> SAPGEDEECGRVRDFVAKLANNTHQHVFDDLRGSVSLSWVGDSTGVILVLTTFHVPLVIMTFGQSKLYRSEDYGKNFKDITDLINNTFIRTEFGMAIGPENSGKVVLTAEVSGGSRGGRIFRSSDFAKNFVQTDLPFHPLTQMMYSPQNSDYLLALSTENGLWVSKNFGGKWEEIHKAVCLAKWGSDNTIFFTTYANGSCKADLGALELWRTSDLGKSFKTIGVKIYSFGLGGRFLFASVMADKDTTRRIHVSTDQGDTWSMAQLPSVGQEQFYSILAANDDMVFMHVDEPGDTGFGTIFTSDDRGIVYSKSLDRHLYTTTGGETDFTNVTSLRGVYITSVLSEDNSIQTMITFDQGGRWTHLRKPENSECDA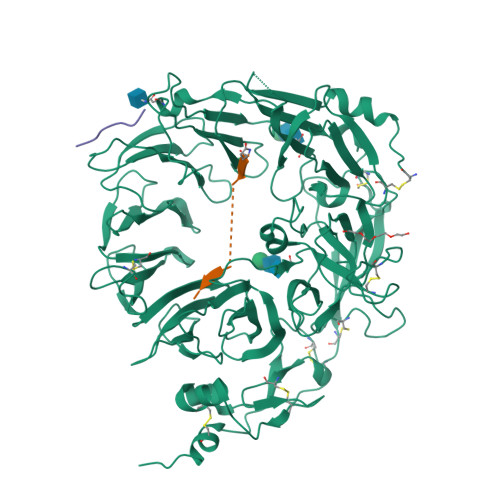TAKNKNECSLHIHASYSISQKLNVPMAPLSEPNAVGIVIAHGSVGDAISVMVPDVYISDDGGYSWTKMLEGPHYYTILDSGGIIVAIEHSSRPINVIKFSTDEGQCWQTYTFTRDPIYFTGLASEPGARSMNISIWGFTESFLTSQWVSYTIDFKDILERNCEEKDYTIWLAHSTDPEDYEDGCILGYKEQFLRLRKSSMCQNGRDYVVTKQPSICLCSLEDFLCDFGYYRPENDSKCVEQPELKGHDLEFCLYGREEHLTTNGYRKIPGDKCQGGVNPVREVKDLKKKCTSNFLSPEKQNSKSNSHHHHHH;>[2x]QLYENKPRRPYIL> SMFLPPPECPVFEPSWEEFADPFAFIHKIRPIAEQTGICKVRPPPDWQPPFACDVDKLHFTPRIQRLNELEAQTRVKLARDYTLRTFGEMADAFKSDYFNMPVHMVPTELVEKEFWRLVSTIEEDVTVEYGADIASKEFGSGFPVRDGKIKLSPEEEEYLDSGWNLNNMPVMEQSVLAHITADICGMKLPWLYVGMCFSSFCWHIEDHWSYSINYLHWGEPKTWYGVPGYAAEQLENVMKKLAPELF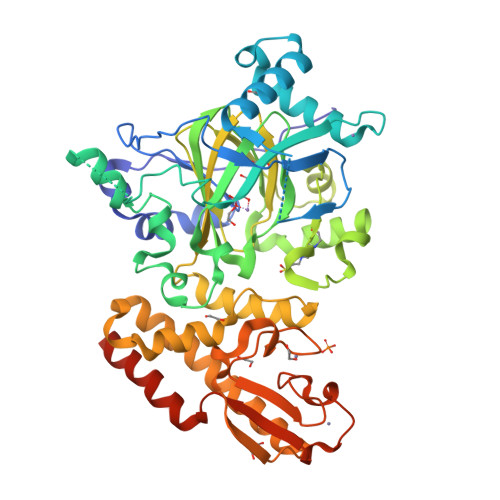VSQPDLLHQLVTIMNPNTLMTHEVPVYRTNQCAGEFVITFPRAYHSGFNQGFNFAEAVNFCTVDWLPLGRQCVEHYRLLHRYCVFSHDEMICKMASKADVLDVVVASTVQKDMAIMIEDEKALRETVRKLGVIDSERMDFELLPDDERQCVKCKTTCFMSAISCSCKPGLLVCLHHVKELCSCPPYKYKLRYRYTLDDLYPMMNALKLRAESYNEWALNVNEALEAKI>MIDYTAAGFTLLQGAHLYAP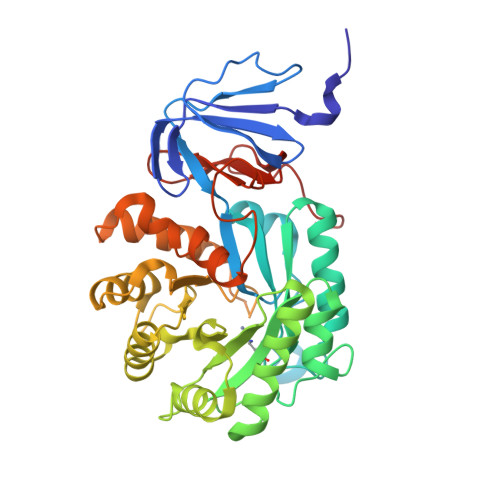EDRGICDVLVANGKIIAVASNIPSDIVPNCTVVDLSGQILCPGFIDQHVHLIGGGGEAGPTTRTPEVALSRLTEAGVTSVVGLLGTDSISRHPESLLAKTRALNEEGISAWMLTGAYHVPSRTITGSVEKDVAIIDRVIGVKCAISDHRSAAPDVYHLANMAAESRVGGLLGGKPGVTVFHMGDSKKALQPIYDLLENCDVPISKLLPTHVNRNVPLFEQALEFARKGGTIDITSSIDEPVAPAEGIARAVQAGIPLARVTLSSDGNGSQPFFDDEGNLTHIGVAGFETLLETVQVLVKDYDFSISDALRPLTSSVAGFLNLTGKGEILPGNDADLLVMTPELRIEQVYARGKLMVKDGKACVKGTFETA[2x]>MTSEQTGEPAEDTSGVIKMAVKFDRRAYPAQITPKMCLLEWCRREKLAQPVYETVQRPLDRLFSSIVTVAEQKYQSTLWDK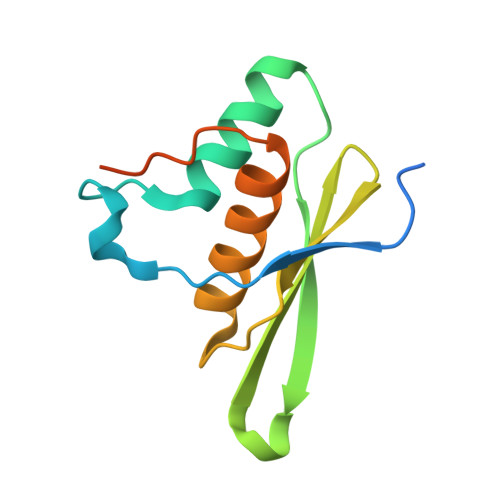SKKLAEQAAAIVCLRSQGLPEGRLGEESPSLHKHHHHHH[3x]> GPLGSPNSQYLKTRILDIYTPEQRAGIEKSEDWRQFSRRMDTHFPKLMNELDSVYGNNEALLPMLEMLLAQAWQSYSQRNSSLKDIDIARENNPDWILSNKQVGGVCYVDLFAGDLKGLKDKIPYFQELGLTYLHLMPLFKCPEGKSDGGYAVSSYRDVNPALGTIGDLREVIAALHEAGISAVVDFIFNHTSNEHEWAQRCAAGDPLFDNFYYIFPDRRMPDQYDRTLREIFPDQHPGGFSQLEDGRWVWTTFNSFQWDLNYSNPWVFRAMAGEMLFLANLGVDILRMDAVAFIWKQMGTSCENLPQAHALIRAFNAVMRIAAPA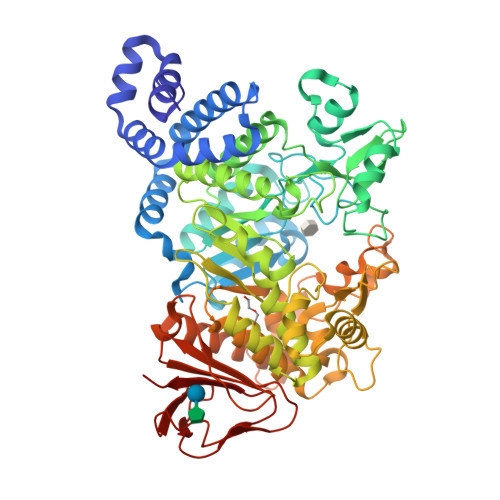VFFKSEAIVHPDQVVQYIGQDECQIGYNPLQMALLWNTLATREVNLLHQALTYRHNLPEHTAWVNYVRSHDDIGWTFADEDAAYLGISGYDHRQFLNRFFVNRFDGSFARGVPFQYNPSTGDCRVSGTAAALVGLAQDDPHAVDRIKLLYSIALSTGGLPLIYLGDEVGTLNDDDWSQDSNKSDDSRWAHRPRYNEALYAQRNDPSTAAGQIYQDLRHMIAVRQSNPRFDGGRLVTFNTNNKHIIGYIRNNALLAFGNFSEYPQTVTAHTLQAMPFKAHDLIGGKTVSLNQDLTLQPYQVMWLEIA> CPSQCSCSGTTVDCRSKRHASVPAGIPTNAQILYLHDNQITKLEPGVFDSLINLKELYLGSNQLGALPVGVFDSL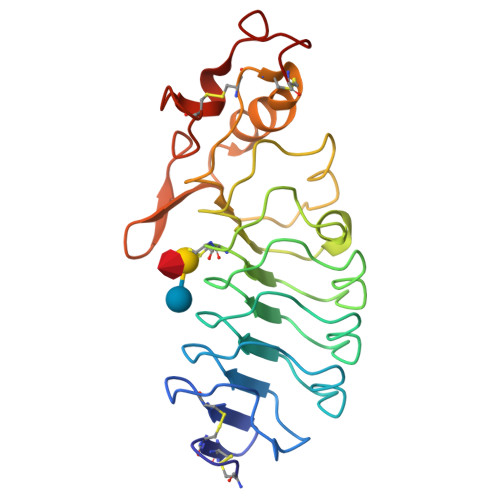TQLTVLDLGTNQLTVLPSAVFDRLVHLKELFMCCNKLTELPRGIERLTHLTHLALDQNQLKSIPHGAFDRLSSLTHAYLFGNPWDCECRDIMYLRNWVADHTSIAMRWDGKAVNDPDSAKCAGTNTPVRAVTEASTSPSKC> AFQETNPPAGPVRAIAEYERSAAVLVRYPFGIPMELIKELAKNDKVITIVASESQKNTVITQYTQSGVNLSNCDFIIAKTDSYWTRDYTGWFAMYDTNKVGLVDFIYNRPRPNDDEFPKYEAQYLGIEMFGMKLKQTGGNYMTDGYGSAVQSHIAYTENSSLSQAQVNQKMKDYLGITHHDVVQDPNGEYINHVDCWGKYLAPNKILIRKVPDNHPQHQALEDMAAYFAAQTCAWGTKYEVYRALATNEQPYTNSLILNNRVFVPVNGPASVDNDALNVYKTAMPGYEIIGVKGASGTPWLGTDALHCRTHEVADKGYLYIKHYPILGEQAGPDYKIEADVVSCANATISPVQCYYRINGSGSFKAADMTMESTGHYTYSFTGLNKNDKVEYYISAADNSGRKETYPFIGEPDPFKFTCMNETNTCTVTGAA

Uniquely among microbes to date, P. gingivalis also produces a secreted PAD (called PPAD18), which protects P. gingivalis during acidic cleansing in the mouth through ammonia generated during host and endogenous protein citrullination. PPAD does not require calcium for catalysis and is genetically unrelated with animal PADs and, like the latter and cysteine peptidases, its main catalytic residue is a cysteine (C351 in PPAD20). In contrast, PPAD citrullinates C-terminal arginines like those generated by the prior action of Rgps17, which may be facilitated by the surface co-localization of Rgps and PPAD20.

We solved three distinct structures to high resolution from different protein preparations, which crystallized in different space groups: substrate-free (to 1.5 Å resolution), a substrate-mimic (1.4 Å), and a substrate complex (1.8 Å). In the substrate-free structure, which was obtained with DTDP-treated wild-type (wt) protein, catalytic C351, nearby C239 and distal C462 residues are covalently modified by what was conservatively interpreted as a 4-thiopyridyl moiety. The C239 side chain is even found in two alternate conformations, one bound to thiopyridine and the other with the sulfur as sulfoxide. This indicates overall flexibility of active site residues in PPAD due to the absence of a bound substrate and suggests that the covalent modifications of the Sγ atoms do not distort the general unbound conformation of PPAD. In addition, segment V226-V237 of the loop connecting blades III and IV, hereafter the “Michaelis loop”, is in an open conformation, thus consistent with a structure that can bind a substrate. In particular, Y233 at the most exposed part of the loop points to bulk solvent. We hypothesize that DTDP-treatment precludes substrate binding and, thus, protects the unbound conformation, while lack of such treatment causes the enzyme to trap substrates or mimics during biosynthesis or purification. In the substrate-free state, the Michaelis-loop containing Y233 is in an open conformation, which enables peptides with a C-terminal arginine to be accommodated at the active site. D130 becomes rotated around its χ1 angle by ~60° upon substrate binding, thereby exchanging its tight hydrogen bond with T180Oγ1 (2.6 Å) in the substrate-free structure with binding of the substrate guanidinium group.>[3x]MGRHYQETQAVEAGEKTVEQFVQALNKGDYNKAAGMASKKAANKSALSEKEILEKYQNIYGAADVKGLEISNLKVDKKDDSTYSFSYKAKMNTSLGELKDLSYKGTLDRNDGKTTINWQPNLVFPEMEGNDKVSLTTQEATRGNILDRNGEPLATTGKLKQLGVVPSKLGDGDEKTANIKAIASAFDLTEDAINQAISQSWVQPDYFVPLKIIDGATPELPAGATIQEVDGRYYPLGEAAAQLIGYVGDITAEDIDKNPELSSNGKIGRSGLEMAFDKDLRGTTGGKLSITDTDGVEKKVLIEHEVQNGKDIKLTIDAKAQKTAFDSLGGKAGSTVATTPKTGDLLALASSPSYDPNKMTNGISQEDYKAYEENPEQPFISRFATGYAPGSTFKMITAAIGLDNGTIDPNEVLT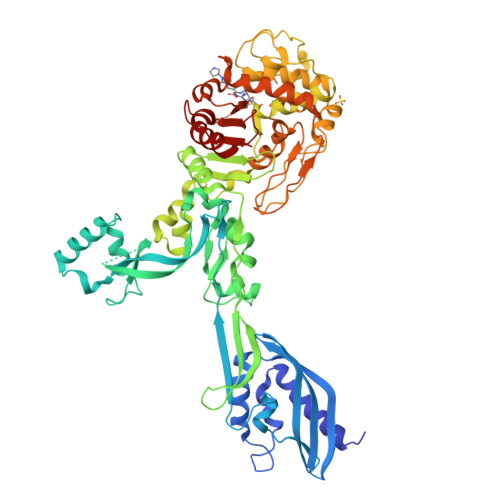INGLKWQKDSSWGSYQVTRVSDVSHVDLKTALIYSDNIYMAQETLKMGEKNFRAGLDKFIFGEDLDLPISMNPAQISNEESFNSDILLADTGYGQGELLINPIQQAAMYSVFANNGTLVYPKLIADKETKDKKNVIGETAVQTIVPDLREVVQDVNGTAHSLSALGIPLAAKTGTAEIKEKQDEKGKENSFLFAFNPDNQGYMMVSMLENKEDDDSATKRAPELLQYLNQNYQLE> MIDLDFRKLTIEECLKLSEEEREKLPQLSLETIKRLDPHVKAFISVRENVSVEKKGKFWGIPVAIKDNILTLGMRTTCASRILEN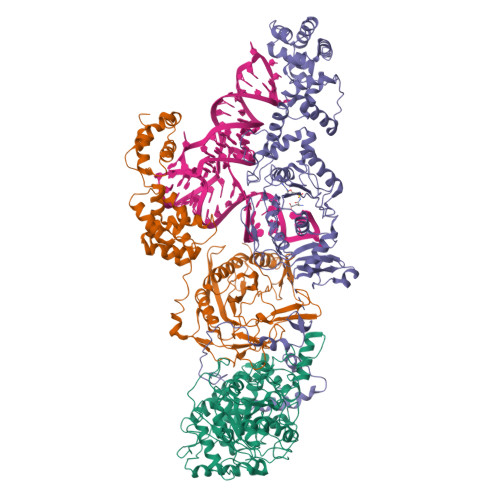YESVFDATVVKKMKEAGFVVVGKANLDEFAMGSSTERSAFFPTRNPWDLERVPGGSSGGSAAAVSAGMVVAALGSDTGGSVRQPASLCGVVGYKPTYGLVSRYGLVAFASSLDQIGPITKTVRDAAILMEIISGRDENDATTVNRKVDFLSEIEEGVSGMKFAVPEEIYEHDIEEGVSERFEEALKLLERLGAKVERVKIPHIKYSVATYYVIAPAEASSNLARFDGVKYGLRIKEKGLREMYMKTRNVGFGEEVRRRIMIGTFTLSAAYYEAYFNKAMKVRRKISDELNEVLSQYDAILTPTSPVTAFKIGEIKDPLTYYLMDIFTIPANLAGLPAISVPFGFSNNLPVGVQVIGRRFADGKVFRIARAIEKNSPYNENGMFPLPEVKA;> MRYRPVIGLEIHVQLSTKTKAFCSCPADVFELPPNTAICPVCTGQPGALPVPNEEMIRFAVKTALALNCKIHKYSRFDRKNYFYPDLPKGYQISQYFYPIATEGFLEIDGDEGRKKVRIRRLHLEEDAGKLVHEGDSITRASYSLVDMNRCGVPLIEIVTEPDISSPREARVFMEKLRSIVRYLGVSTGDMEKGALRCDANISVVDTETGRQSNRVEVKNMNSFRFVERALEYEFERIVKAMERGEDVERETRGWDMATKITVSMRGKEEESDYRYFPEPDIPPVVLSDEYLEEVKKELPELPDEKAERFMREYGLPEYDAKVLTSSKELAEFFEECVKVVNRPKDLSNWIMTEVLRELNERNIEITESKLTPQHFADLFKLMDEGKISIKIAKEIFPEVFETGKMPSQIVEEKGLTQINDEKLIEELVKKAMEQNPKAVQDYKSGKKKAAGFFVGYVMRETKGKANPELTNRIIQKLLEGE;> MGIKVTKDLVLHLENLARLELSEDQRESLMKDFQEILDYVELLNEVDVEGVEPMYTPVEDSAKLRKGDPRFFEMRDLIKKNFPEEKDGHIKVPGIHRGSGSGSGSMFITGAFFDILEVGPKKIRRCFELVRVRFAPSPTGHLHVGGARTALFNWMFARKEGGKFILRIEDTDTERSSREYEQQILESLRWCGLDWDEGPDIGGDFGPYRQSERLEIYREYAEKLVEDKRAYYVVYDKEDPSKELFTTYEYPHEYKEKGHPVTIKFKVLPGKTSFEDLLKGYMEFDNSTLEDFIIMKSNGFPTYNFAVVVDDHLMRISHVFRGEDHLSNTPKQLMIYEAFGWEAPVFMHIPLILGSDRTPLSKRHGATSVEHFRREGILSRALMNYLALLGWRVEGDEIFTIEEKLQSFDPKDISNKGVIFDYQKLEWVNGKHMRRIDLEDLKREFIEWAKYAGKEIPSVDERYFSETLRICREKVNTLSQLYDIMYPFMNDDYEYEKDYVEKFLKREEAERVLEEAKKAFKDLNSWNMEEIEKTLRDLSEKGLASKKVVFQLIRGAVTGKLVTPGLFETIEVLGKERTLKRLERTLQFLKKT> MSKSKMIVRTKFIDRACHWTVVICFFLVALSGISFFFPTLQWLTQTFGTPQMGRILHPFFGIAIFVALMFMFVRFVHHNIPDKKDIPWLLNIVEVLKGNEHKVADVGKYNAGQKMMFWSIMSMIFVLLVTGVIIWRPYFAQYFPMQVVRYSLLIHAAAGIILIHAILIHMYMAF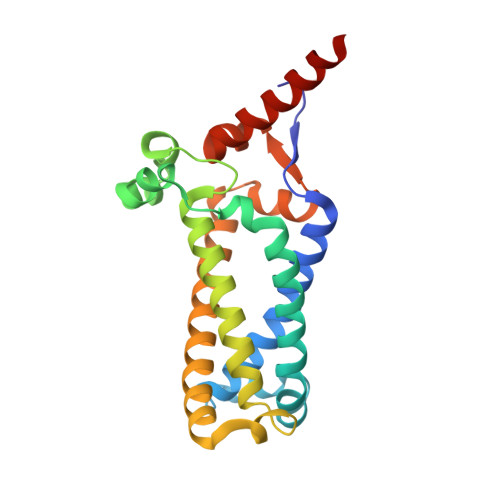WVKGSIKGMIEGKVSRRWAKKHHPRWYREIEKAEAKKESEEGI> FSVLNWDQVSRLHEVLTEVVPIHGRGNFPTLEITLKDIVQTVRS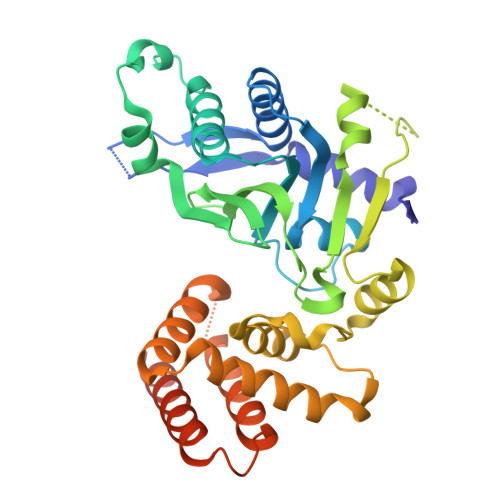RLEEAGIKVHDVRLNGSAAGHVLVKDNGLGCKDLDLIFHVALPTEAEFQLVRDVVLCSLLNFLPEGVNKLKISPVTLKEAYVQKLVKVCTDTDRWSLISLSNKNGKNVQLKFVDSIRRQFEFSVDSFQIILDSLLDFYDCSNNPISEHDHPTVIGESMYGDFEEAFDHLQNRLIATKNPEEIRGGGLLKYSNLLVRDFRPTDQEEIKTLERYMCSRFFIDFPDILEQQRKLETYLQNHFAEEERSKYDYLMILRRVVNESTVCLMGHERRQTLNLISLLALRVLAEQNIIPSATNVTCYYQ>[7x]MGATRIQAVYRDTGVEAYRDNPFIEALPPLQESVNSAASLKSSLQLTSSDLQKSRVIRAHTICRIPDDYFQPLGTHLLLSERISVMIRGGYVGRNPKTGDLQKHLQNGYERVQTGELETFRFEEARSTAQSLLLIGCSGSGKTTSLHRILATYPQVIYHRELNVEQVVYLKIDCSHNGSLKEICLNFFRALDRALGSNYERRYGLKRHGIETMLALMSQIANAHVLGLLVIDEIQHLSRSRSGGSQEMLNFFVTMVNIIGVPVMLIGTPKAREIFEADLRSARRGAGFGAIFWDPIQQTQRGKPNQEWIAFTDNLWQLQLLQRKDALLSDEVRDVWY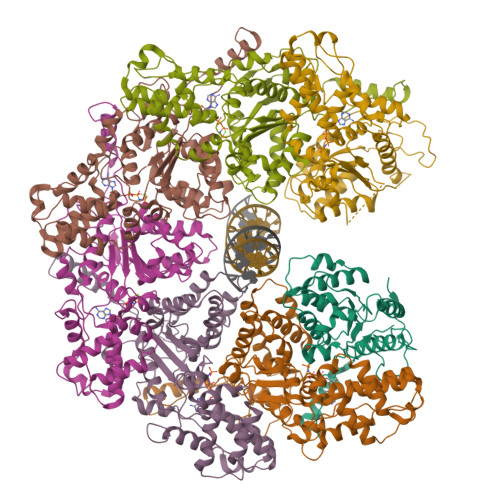ELSQGVMDIVVKLFVLAQLRALALGNERITAGLLRQVYQDELKPVHPMLEALRSGIPERIARYSDLVVPEIDKRLIQLQLDIAAIQEQTPEEKALQELDTEDQRHLYLMLKEDYDSSLLIPTIKKAFSQNPTMTRQKLLPLVLQWLMEGETVVSELEKPSKSKKVSPNSSSVDKLAAALEHHHHHH>MIIRDVELVKVARTPGDYPPPLKGEVAFVGRSNVGKSSLLNALFNRKIAFVSKTPGKTRSINFYLVNSKYYFVDLPGYGYAKVSKKERMLWKRLVEDYFKNRWSLQMVFLLVDGRIPPQDSDLMMVEW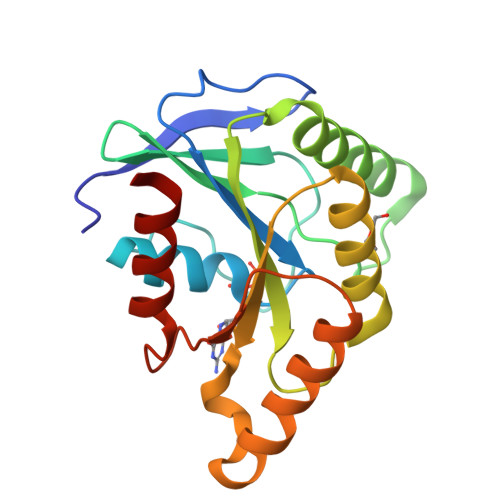MKSLNIPFTIVLTKMDKVKMSERAKKLEEHRKVFSKYGEYTIIPTSSVTGEGISELLDLISTLLKEN[2x]> GGAGAGATGTGCGGAGATAATCAGCTTTTTATATGTGAAAAGGCCGTTTTTACCAATAGATCAGATTGGTCATTTTCG;> CGAAAATGACCAATCTGATCTATTGGTAAAAACGGCCTTTTCACATATA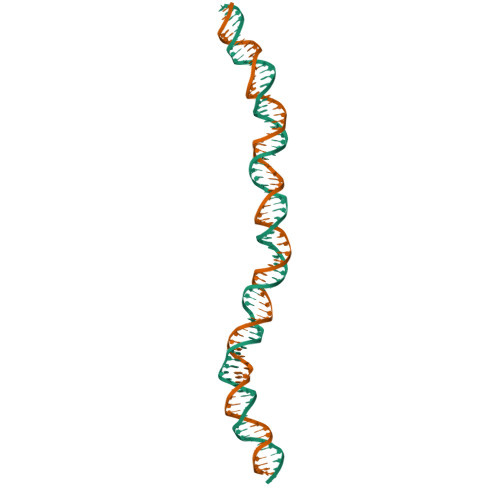AAAAGCTGATTATCTCCGCACATCTCTCC>[4x]MLS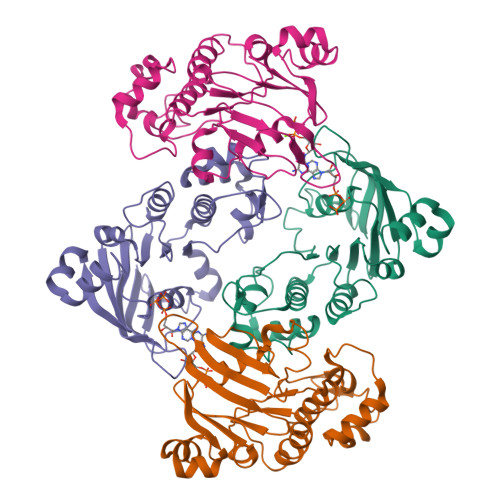ARHVDFAYDDSEQILRDISFEAQPNSIIAFAGPSGGGKSTIFSLLERFYQPTAGEITIDGQPIDNISLENWRSQIGFVSQDSAIMAGTIRENLTYGLEGDYTDEDLWQVLDLAFARSFVENMPDQLNTEVGERGVKISGGQRQRLAIARAFLRNPKILMLDEATASLDSESESMVQKALDSLMKGRTTLVIAHRLSTIVDADKIYFIEKGQITGSGKHNELVATHPLYAKYVSEQLTVGQ> MSGSFWTSTQRHHWQYTKASLAKERQKLWLLECQLFPQGLNIVMDSKQNGIEQSITKNIPITHRDLHYDKDYNLRIYCYFLIMKL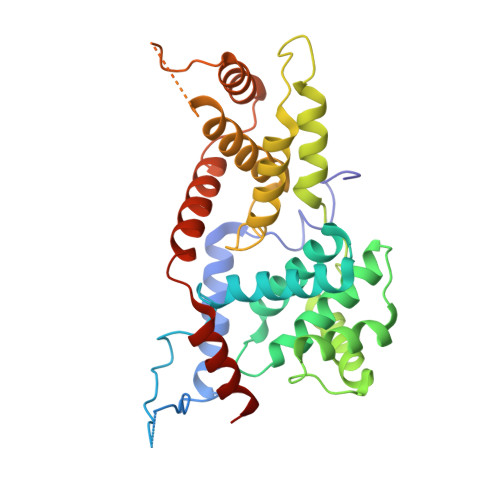GRRLNIRQYALATAHIYLSRFLIKASVREINLYMLVTTCVYLACKVEECPQYIRTLVSEARTLWPEFIPPDPTKVTEFEFYLLEELESYLIVHHPYQSLKQIVQVLKQPPFQITLSSDDLQNCWSLINDSYINDVHLLYPPHIIAVACLFITISIHGKPTKGSSLASAASEAIRDPKNSSSPVQIAFNRFMAESLVDLEEVMDTIQEQITLYDHWDKYHEQWIKFLLHTLYLRPASAI> MPFGKPLVGTLLASLTLLGLATAHAKDDMKAAEQYQGAASAVDPAHVVRTNGAPDMSESEFNEAKQIYFQRCAGCHGVLRKGATGKPLTPDITQQRGQQYLEALITYGTPLGMPNWGSSGELSKEQITLMAKYIQHTPPQPPEWGMPEMRESWKVLVKPEDRPKKQLNDLDLPNLFSVTLRDAGQIALVDGDSKKIVKVIDTGYAVHISRMSASGRYLLVIGRDARIDMIDLWAKEPTKVAEIKIGIEARSVESSKFKGYEDRYTIAGAYWPPQFAIMDGETLEPKQIVSTRGMTVDTQTYHPEPRVAAIIASHEHPEFIVNVKETGKVLLVNYKDIDNLTVTSIGAAPFLHDGGWDSSHRYFMTAANNSNKVAVIDSKDRRLSALVDVGKTPHPGRGANFVHPKYGPVWSTSHLGDGSISLIGTDPKNHPQYAWKKVAELQGQGGGSLFIKTHPKSSHLYVDTTFNPDARISQSVAVFDLKNLDAKYQVLPIAEWADLGEGAKRVVQPEYNKRGDEVWFSVWNGKNDSSAL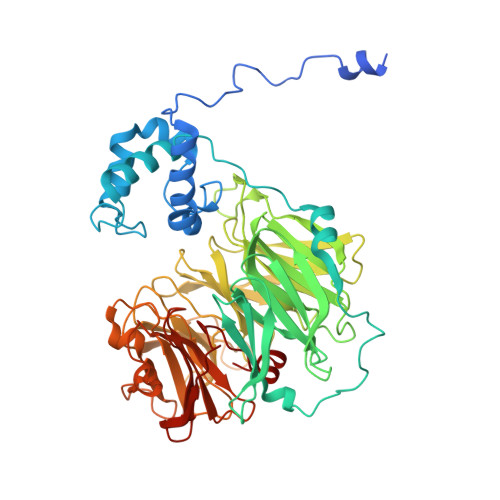VVVDDKTLKLKAVVKDPRLITPTGKFNVYNTQHDVY>[2x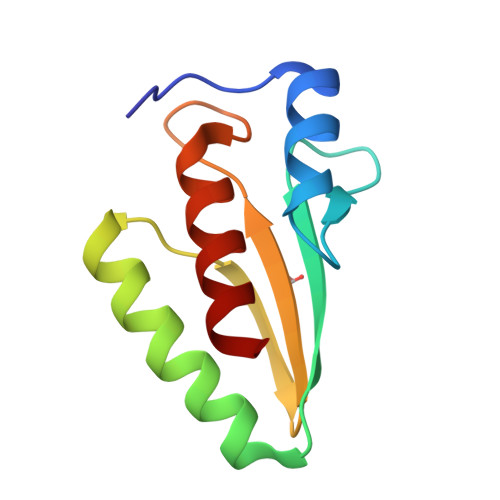]MARNRLTESEMNEALRALDGWQKVDGREAITRSFKFKDFSTAFGFMAQAALYAEKLDHHPEWFNAYNRVDVTLATHSENGVTELDIKMARKMNAIAG Torsins are essential proteins that belong to the AAA + (ATPases associated with a variety of cellular activities) superfamily. Torsins are restricted to multicellular eukaryotes and they exclusively reside in the endoplasmic reticulum (ER) and the connected perinuclear space (PNS). From a medical perspective TorsinA is important, since a deletion of glutamate 303 in TorsinA, TorsinAΔE for short, is the founding mutation for early-onset primary dystonia, a devastating and still incurable neuromuscular movement disorder. While LAP1 and LULL1 provide the Arg finger for activating ATP hydrolysis, they are unable to bind nucleotide themselves, due to a lack of the characteristic sequence motifs introduced above.

Proteolytically cleaving MBP with 3C protease, combined with ATP-containing buffer resulted in longer filaments, which were then suitable for helical reconstruction. The resulting structure showed TorsinA to assemble into a helical filament with an outer diameter of ~14.5 nm. Surprisingly, and in contrast to most AAA + ATPases, we observe that the filament has a central channel with a diameter of ~4 nm. The filaments have a right-handed 1-start helix with a pitch of ~47 Å, and they contain 8.5 TorsinA molecules per turn with an axial rise of 5.5 Å per subunit. The EM density for the small domain of TorsinA is less well defined than the large domain, potentially indicating some flexibility. The superposition of filamentous TorsinA with its heterodimeric LULL1-bound state18 shows that the protein rearranges significantly. There, the rearrangement of residues 232–262, is critical to prevent steric clashes with the nucleotide bound to the neighboring unit. We presume that the TorsinA filaments are nucleotide bound for two reasons: first, we observed EM density at the nucleotide-binding site, and second, we observed robust filament formation only in ATP-containing buffer. We performed an NADH-coupled ATPase assay and observed no ATPase activity. The electrostatic surface along the inner channel of TorsinA shows an undulating pattern of positively and negatively charged stripes.

>GQKRSLSREALQKDLDDNLFGQHLAKKIILNAVFGFINNPKPKKPLTLSLHGWTGTGKNFVSKIIAENIYEGGLNSDYVHLFVATLHFPHASNITLYKDQLQLWIRGNVSACARSIFIFDEMDKMHAGLIDAIKPFLDYYDLVDGVSYQKAMFIFLSNAGAERITDVALDFWRSGKQREDIKLKDIEHALSVSVFNNKNSGFWHSSLIDRNLIDYFVPFLPLEYKHLKMCIRVEMQSRGYEIDEDIVSRVAEEMTFFPKEERVFSDKGCKTVFTKLDYYYDD[25x]> MASMTGGQQMGRDEAGITGTWYNQLGSTFIVTAGADGALTGTYESAVGNAESRYVLTGRYDSAPATDGSGTALGWTVAWKNNYRNAHSATTWSGQYVGGAEARIN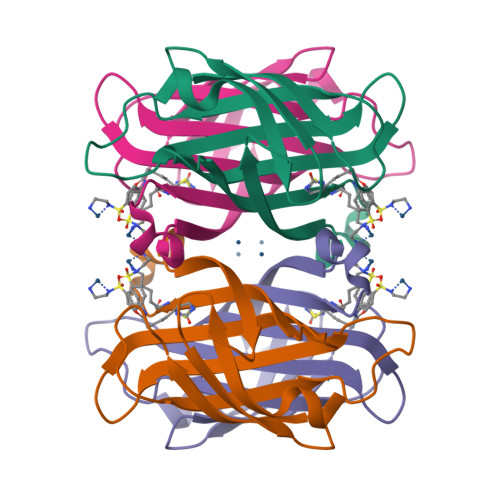TQWLLTKGTTEANAWKSTLVGHDTFTKVKPSAASIDAAKKAGVNNGNPLDAVQQ In the initial step, phosphatidylinositol-phosphate (PIP) synthases generate PIP using L-myo-inositol-1-phosphate (inositol phosphate) as the acceptor alcohol and CDP-DAG as the donor substrate; subsequently, the terminal phosphate is removed by an as-yet-unidentified phosphatase to yield PI4. All (class I) CDP-APs are integral membrane enzymes that catalyse the transfer of a substituted phosphate group from a CDP-linked donor, CDP-DAG for PI and PIP biosynthesis, to an acceptor alcohol to generate a phosphodiester-linked product. We have determined the crystal structures of PIP synthase from Renibacterium salmoninarum, in the apo form and with bound CDP-DAG to 2.5 and 3.6 Å resolution, respectively. RsPIPS adopts a homodimeric architecture similar to those previously observed in Af2299 and AfDIPP synthase, with each protomer possessing six TM helices surrounding a large polar cavity.

We determined the structure of a chimeric construct of PIP synthase from R. salmoninarum (RsPIPS)—the causative agent for bacterial kidney disease in salmonids, a major threat to these species worldwide17—in which the first six residues of the RsPIPS sequence were omitted (RsPIPS-Δ6N). Crystals of RsPIPS-Δ6N diffracted X-rays to 2.5 Å resolution, and the structure was solved by molecular replacement using the cytidylyltransferase-like domain of Af2299 as a search model. The crystals of RsPIPS-Δ6N diffracted well in the apo-state (2.5 Å), but attempts to obtain co-crystal structures with CDP-DAG were unsuccessful. In RsPIPS, the central polar cavity is located at the cytosolic boundary of the membrane, and contains three distinct regions, which together form the active site. Proximal to the nucleotide-binding site, and within the membrane-spanning region is a pocket wedged between TMs 4, 5 and 6, which probably represents the inositol phosphate acceptor-binding cavity. Several conserved residues line this cavity, including two arginine residues (R153 and R191) that in the structure of RsPIPS-Δ6N coordinate a ion present at high concentration in the crystallization solution. We hypothesize that these residues coordinate the phosphate of inositol phosphate, a moiety unique to PIP synthases. Directly above the nucleotide-binding site, we observed a gap between JM1 and TM2, creating a hydrophobic groove that is open to the membrane. We hypothesize that this diminished activity of MtPIPS-Δ6N is due to compromised binding of CDP-DAG, as JM1 is truncated and distorted in RsPIPS-Δ6N, potentially interfering with CDP-DAG binding. This could provide an explanation as to why we were unable to obtain the structure of RsPIPS-Δ6N in complex with its cognate lipid substrate.

> MRLAYVKNHEIYGEKLLGLTLRERIEKTLQRAGFDVRFFDELSLEEAEDYLIILEPVLILERDLLLEGRKILVSDGFTVGYFFGGDFRTVFDGNLQSSIEKYLSLNNLESYEIWAIKLSNDNLKTAEKLLLSSLIGSRGLFAAIFLPIARLLADWGVSPDAVTVVGTLGVMAGALIFYPMGQLFWGTVVITVFVFSDIIDGLMARLLFREGPWGAFLDSYLDRVGDSSVFTGIVIWFFLGGANPTIAILALICLVLSSLVSYSKARAEGLGLTANVGIAERSERLVVVLVATGLVGLGIPSWVLLVVLIVLAIASVVTIFQRVLTVREQAKAWTAS>[8x]MIGRLRGTLAEKQPPHLILDVNGVGYEVEVPMTTLYRLPSVGEPVTLHTHLVVREDAHLLYGFAEKRERELFRELIRLNGVGPKLALALMSGLEVDELVRCVQAQDTSTLVKIPGVGKKTAERLLVELKDRFKAWEN

Holliday junction (HJ) is a four-way structured DNA intermediate in homologous recombination. In bacteria, the HJ-specific binding protein RuvA and the motor protein RuvB together form the RuvAB complex to catalyze HJ branch migration. During homologous recombination, the RuvB hexameric motors are attached to the RuvA-HJ core complex through the interactions with RuvA domain IIIs (RuvAD3) and thereby drive HJ branch migration and strand exchange between the two homologous DNAs (Iype et al., 1994; Iype et al., 1995; Adams and West, 1996; Wald et al., 2022). Here, we describe the cryo-Electron Microscopy (cryo-EM) structure of the RuvAB-HJ intermediate complex from P. aeruginosa.

The cryo-EM structure of PaRuvA-HJ region was determined at 3.0 Å with well-defined electron density. In agreement with the previous crystal structures of HJ-bound octameric RuvA from Mycobacterium leprae (M. leprae, Ml) (Roe et al., 1998), each PaRuvA subunit is composed of three distinct domains: D1, D2 and D3. The HJ molecule is sandwiched by two PaRuvA tetramers that dimerize through a pair of antiparallel helices, involving at least four pairs of electrostatic interactions and one pair of hydrophobic interaction. The two tetramers together enclose a cross-shaped tunnel of ~ 23 Å in diameter, which encircles ~ 10 bp of HJ arm. The protein-DNA contacts at each HJ arm are mainly mediated by the RuvAD2 and DNA phosphodiester backbone. Interestingly, all RuvAD2 in tetramer 1 insert into the DNA major groove, whereas the equivalent domains in tetramer 2 all bind the minor groove. As a result, the two tetramers do not form a perfect two-fold symmetry but are misaligned by ~18°. The junction center is devoid of base pairs but occupied by a conserved ‘RED’ motif (R54, E55 and D56) in RuvAD1. In the motif, R54 binds to the ribose-phosphate backbone of the branch site with its positively charged guanidino group, while the carboxyl groups of E55 and D56 may provide strong negatively electrostatic repulsion for strand separation. Of note, the base pairs at the branch sites of RuvB-free HJ arms are disrupted and interact with D56, whereas the equivalent base pairs at RuvB-bound arms remain intact.>[8x]GQNHHEVVKFMDVYQRSYCHPIETLVDIF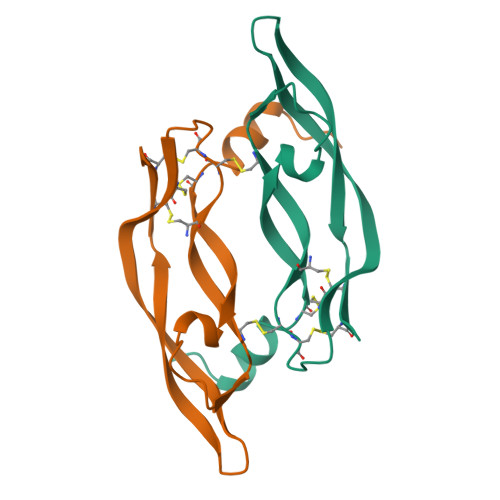QEYPDEIEYIFKPSCVPLMRCGGCCNDEGLECVPTEESNITMQIMRIKPHQGQHIGEMSFLQHNKCECRPKKD> GPLGSEDDLEVKEENGVLVLNDANFDNFVADKDTVLLEFYAPWCGHCKQFAPEYEKIANILKDKDPPIPVAKIDATSASVLASRFDVSGYPTIKILKKGQAVDYEGSRTQEEIVAKVREVSQPDWTPPPEVTLVLTKENFDEVVNDADIILVEFYAPWCGHCKKLAPEYEKAAKELSKRSPPIPLAKVDATAETDLAKRFDVSGYPTLKIFRKGRPYDYNGPREKYGIVDYMIE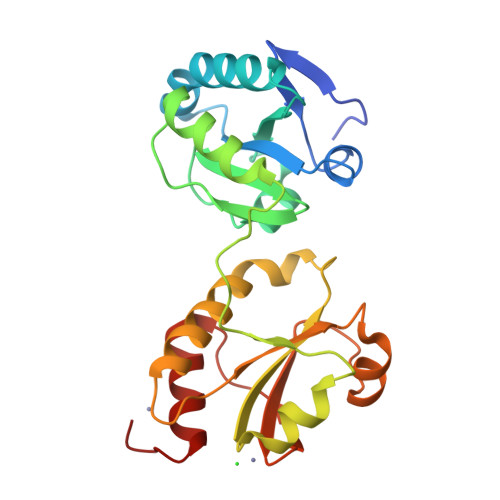QSGAAAS>MSEPFEIVAGALGVAGLFNNCVACFEYVQLGRHFGRDYERCQLRLDIAKVRLSRWGEAVQINDDPRFHSSAPIDKSVQLAKSIVEEILLLFESAQKTSKRYELVADQQDLVVFEDKDMKPIGRALHRRLKDLVSRRQKQTSLAKKTAWALYDGKSLEKIVDQVAGFVDELEKAFPIEAVCHKLAENEIEEVEDEASLTILKDAAGGIDAAMSDAAAQKIDAIVGRNSHHHHH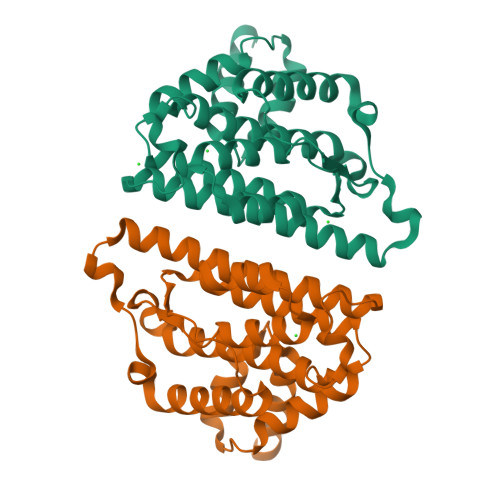H[2x]> MASMTGGQQMGAPITAYAQQTRGLLGCIITSLTGRDKNQVEGEVQIVSTATQTFLATCINGVCWTVYHGAGTRTIASPKGPVIQMYTNVDQDLVGWPAPQGSRSLTPCTCGSSDLYLVTRHADVIPVRRRGDSRGSLLSPRPISYLKGSSGGPLL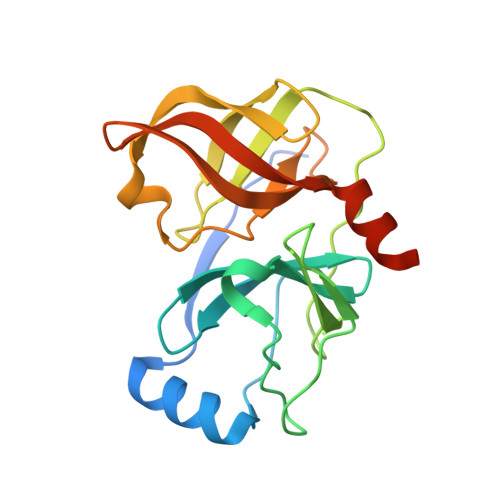CPAGHAVGLFRAAVCTRGVTKAVDFIPVENLETTMRSGSHHHHHH> LRRRVSATPSLAVSPAGPSSLSLTPSPADSQQRRSLKTLDVREYRPLGTPIEFRFYQRYANHPNRQSGVQFLTHYNTHQRFRVNKDFIDYMHWGKEQGQARLPHRHQRVAFDFDDSLQPTRAEGAVGAWFAGQDPTMRSHPDISASFDPNKKLFSHPEHWNKMFSKRRPGEGDIKLNVIPSNSLLGPMVTQTDTQDMAYFKTETCGPTHGRVPGINAPFKGEMDRKMMQAMSRPLNRSCTLTGNNGRFSNTIFINDPKRHQTLSATLAKELNREVDRATN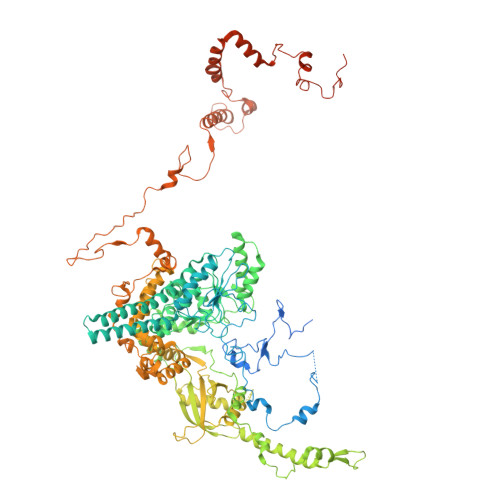GLYSKLTVLTSAQSGLTDFFCGGTDLQCIGFDLTMAQLLRKEADALTKSAASGSKKVEAKVHELLRDAERYEERADSVLRENAAVIWRAYTSPRALMTLVNGKCRGTGCGLALAAKYAGLQDASEFIVDGPNVGLTPYSGMTRLLARPETSLKYPGLAEFVMLTGASLFAGDALRLGWSDLFTSLPDMPYHIKDWFDSTEHMHNDAVAWQLGHLLEKCFQMKDRWHTSAMERCAMTPIRARWVEDAFADQSSIEEILKTLSAMEKLPLTDRHNTYDPSYATPYTLASVAEGVEKLGASRLRYTLSPWDATPPEEAVEVRQAAEIFTSYVLERRGKVNIVAHRDRHKVQAWQKQREREYVAYSNMKNAPHRRHVYVRLEGCEGTLVDFDFTIDPAGDAAAAAAEKGAGVDDRNELVHTASVERLKRAVLQAMGMPADRDVDLCWYLPTLDTCPIRNDEELVDVLHSDPGFEDPSAQLRYPPIYFLVKRNTLHLSEWAYAVKHQLLLQSPYALKATLQLLQEVRGDGSAKAVRSLADTLATEYRYAARLLKRPDFYQVGQHVDKSPEEWDVVKEERMRYVHKAHLPTRPLPDYEVVFERNVQLDGHTFQLRPRWSPRTVQEVTAESLAPLATPLDFEKDGAVEFNVVVHASKADRLAGMIEDAGGFEVVAHLGEVDKEGNAKVPPLHGDAHVPTNVNFYEMARHPWEDTPSSTRRDGFTAGSKEYFEQQYKKAEKAVYDEAGRGQRNYWPSKAAVDGVTGEESNALLEERFFAKLRDAERGVESWARQLRKKAVEGKLDNKPEIATQQEKIYDDDYYRWFIQPGHNPNPSGLLRGRKVADSGSSSVDKDLEVFLNQLLSGAAERGADGTTGDEGEALSLPEEDTDEAADST Protein fem‐1 homolog B (FEM1B) is a substrate recognition protein of the Cullin‐RING (CUL2) E3 ligase and plays a critical role in regulating proteins in the cell (Chen et al., 2021, 2024; Hughes et al., 2021; Kramer & Zhang, 2022; Manford et al., 2021; Raiff et al., 2025; Zhao et al., 2021). FEM1B plays a crucial role in balancing the reductive stress response in the cell by degrading key proteins involved in redox sensing and management (Manford et al., 2021). FEM1B binds multiple degron substrates with distinct recognition sequences, which suggests FEM1B has multiple recognition sites for substrate binding. Here, we describe the development of a stable construct of FEM1B, the results of a protein‐observed NMR‐based fragment screen using this construct, and the X‐ray structures of some of the fragment hits when bound to the protein.

The X‐ray structures were determined for six additional molecules (VU0412674, VU0417412, VU0421763, VU0023775, VU0081201, and VU0432623) in complex with FEM1B. The six additional molecules which are classified as chemical shift pattern 3 sit in the same binding pocket. The other six fragments bound to the same site in the FEM1B substrate binding pocket, a region typically important for identifying C‐terminal prolines of degron substrates in a non‐covalent manner. When the most potent non‐covalent molecules, VU0412674 (KD = 0.26 mM) and VU0417412 (KD = 0.28 mM), are bound to FEM1B, Tyr84 forms a polar contact with the amide carbonyl of the molecules. This, along with Phe130, causes this portion of the binding pocket to “close,” locking the fragments in place. The position of Y84 appears to have a significant impact, with the “closed” position providing an increase in binding affinity by locking the molecule in place.

>GHMEGLAGYVYKAASEGKVLTLAALLLNRSESDIRYLLGYVSQQGGQRSTPLIIAARNGHAKVVRLLLEHYRVQTQQTGTVRFDGYVIDGATALWCAAGAGHFEVVKLLVSHGANVNHTTVTNSTPLRAACFDGRLDIVKYLVENNANISIANKYDNTCLMIAAYKGHTDVVRYLLEQRADPNAKAHCGATALHFAAEAGHIDIVKELIKWRAAIVVNGHGMTPLKVAAESCKADVVELLLSHADCDRRSRIEALELLGASFANDRENYDIIKTYHYLYLAMLERFQDGDNILEKEVLPPIHAYGNRTECRNPQELESIRQDRDALHMEGLIVRERILGGGGSGGGSKKRLLLGLDR[2x]> ANLRLSEANSGTYKTFIGRVREELGSETYRLYGIPV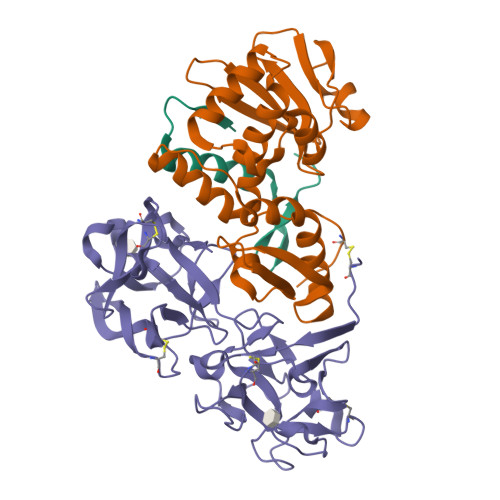LKHSL;> NRFYLLTLTSNKDESITLAIDVEDMVAVAYQPAGSHESYFFLNAPQLAFHTLFTDTHQNVLNFDNTFKSLENAAGTTRQTIVLGVDPLDFAISNLFNADPKLLPLSFLVIIQMVLEASKFRFIEQSVAYSFKNEKTFIPDLAIVSLEDNWSEISLQIQASTSLQGLFGSVVELYNSNNELIEVDSIYYPIILANVALQLYHCQVST;> NECIVETRTTRISGRDALCVDVAGALTSDGSRLILYPCGQQVNQKWTFHSDGTVRSLGKCLATNNSKFGNLVVIYDCSKLAAEDISWDVSVGGTIMNPNYEDLALTSNKATRSTNLTMEVNTYSASQGWRVGNYVQPIIGSIVGLDDMCLEATDGNTNMWLEECVPNKREQSWALYSDGTIRVDDNRELCVTASSSTYDNWKVITILNCDGSNNQRWVFLADGSISTPGNQRLAMDVARSDVDLKKIILHRPHGDLNQQWVLFY> MGGGGTDRVRRSEAIT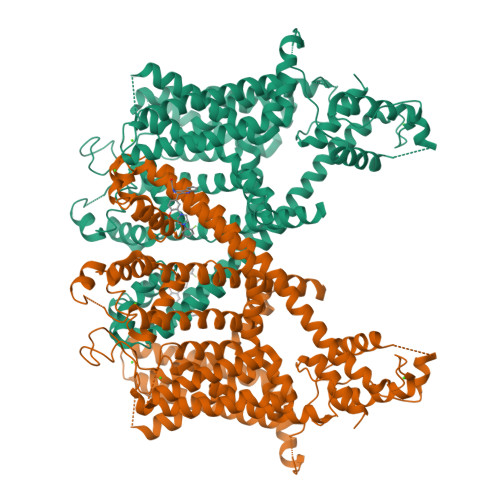HGTPFQKAAALVDLAEDGIGLPVEILDQSSFGESARYYFIFTRLDLIWSLNYFALLFLNFFEQPLWCEKNPKPSCKDRDYYYLGELPYLTNAESIIYEVITLAILLVHTFFPISYEGSRIFWTSRLNLVKVACVVILFVDVLVDFLYLSPLAFDFLPFRIAPYVRVIIFILSIRELRDTLVLLSGMLGTYLNILALWMLFLLFASWIAFVMFEDTQQGLTVFTSYGATLYQMFILFTTSNNPDVWIPAYKSSRWSSVFFVLYVLIGVYFVTNLILAVVYDSFKEQLAKQVSGMDQMKRRMLEKAFGLIDSDKNGEIDKNQCIKLFEQLTNYRTLPKISKEEFGLIFDELDDTRDFKINKDEFADLCQAIALRFQKEEVPSLFEHFPQIYHSALSQQLRAFVRSPNFGYAISFILIINFIAVVVETTLDIEESSAQKPWQVAEFVFGWIYVLEMALKIYTYGFENYWREGANRFDFLVTWVIVIGETATFITPDENTFFSNGEWIRYLLLARMLRLIRLLMNVQRYRAFIATFITLIPSLMPYLGTIFCVLCIYCSIGVQVFGGLVNAGNKKLFETELAEDDYLLFNFNDYPNGMVTLFNLLVMGNWQVWMESYKDLTGTWWSITYFVSFYVITILLLLNLVVAFVLEAFFTELDLEEEEKCQGQDSQEKRNRRRSAGSKSRSQRVDTLLHHMLGDELSKPECSTSDTLVPR(3~{R},4~{R})-4-[4-[(5-bromanylpyridin-3-yl)oxymethyl]-1,2,3-triazol-1-yl]pyrrolidin-3-ol 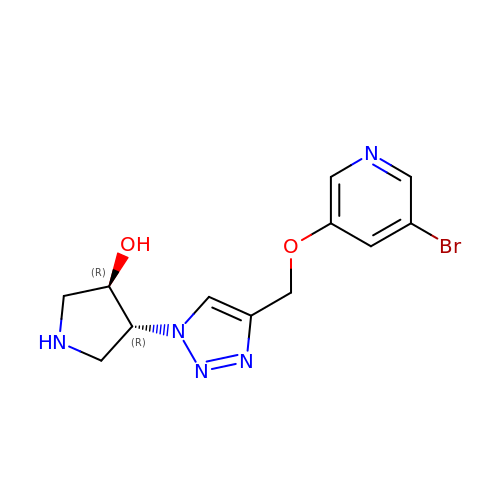| C12 H14 Br N5 O2 | GZDISGCMSVDHKR-VXGBXAGGSA-N>GSPGISGGGGGILSLLCVGVKKAKFDGAQEKFNTYVTLKVQNVESTTIAVRGSQPSWEQDFMFEINRLDLGLTVEVWNKGLIWDTMVGTVWIPLRTIRQSNEEGPGEWLTLDSQAIMADSEICGTKDPTFHRILLDAHFELPLDIPEEEARYWAKKLEQLNAKLNSS[2x];> GSQEQKGDAPTCGICHKTKFADGCGHNCSYCQTKFCARCGGRVSLRSNKVMWVCNLCRKQ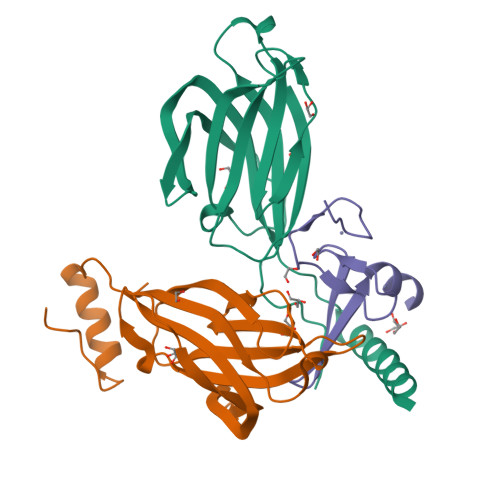QE> MTKKVGLLVMAYGTPYKDEDIERYY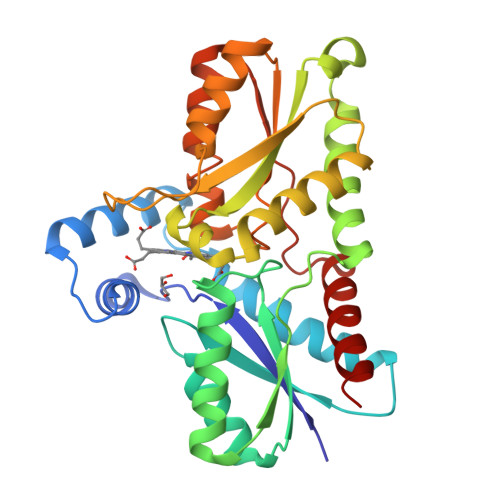TDIRHGHKPSEEMIADLRGLYHAIGGLSPLAKITEAQAYGLEKALNDSQDEVEFKAYIGLKHIEPFIEDAVEAMHKDGIEEAISIVLAPHYSSFSVEAYNKRAKEAADKLGGPRINAINDWYKQPKFIQMWADRINETAKQIPADELLDTVLIVSAHSLPEKIKQHNDPYPNQLQETADFIFEKVVVPHYALGWQSEGKTGEPWLGPDVQDLTRELYGREKYKHFIYTPVGFVAEHLEVLYDNDYECKVVTDEVGAAYHRPPMPNSDPEFLEVLRTVVWEKYSNLE> MTDKLIRELLIDVKQKGATRTAKSIENVSDALENAAAASE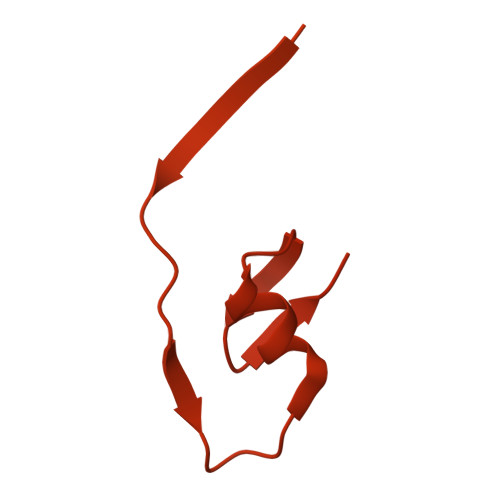LTNEQLGKMPRTLYSIERAADRAAKSLTKMQASRGMAGITKSIDGIGDKLDYLAIQLIEVTDKLEIGFDGVSRSVKAMGNDVAAATEKVQDRLYDTNRALGGTSKGFNDTAGAAGRASRALGNTSGSARGATRDFAAMAKIGGRLPIMYAALASNVFVLQTAFESLKVGDQLNRLEQFGTIVGTMTGTPVQTLALSLQNATNGAISFEEAMRQASSASAYGFDSEQLEQFGLVARRAAAVLGVDMTDALNRVIKGVSKQEIELLDELGVTIRLNDAYENYVKQLNATSTGIKYTVDSLTTYQKQQAYANEVIAESTRRFGYLDDALKATSWEQFAANANSALRSLQQSAATYLNPVMDTLNTFLYQTKSSQMRVSAMARSASAKTTPAENVTALIENAVGAREDLDTYLKESEERVKKAQELKQQLDDLKAKQAATAPIANALTAGGIGGDESNKLVVQLTNELARQNKEIEERTKTEKVLRQAVQDTGEALLRNGKLAEQLGAKMKYADTAVPGDKGVFEVDPNNLKAVSEIQKNFDFLKKSSSDTANNIRMAASSITNAKKASSDLNSVVKAVEDTSKVTGQSADTLVKNLNLGFSSLDQMKAAQKGLSEYVTAMDKSEQNALEVAKRKDEVYNQTKDKAKAEAAAREVLLRQQQEQLTAAKALLAINPNDPEALKQVAKIETEILNTKAQGFENAKKTKDYTDKILGVDREIALLNDRTMTSTQYRLAQLRLELQLEQEKTELYSKQADGQAKVEQSRRAQAQISREIWEAEKQGTASHVSALMDALEVSQTQRNVTGQSQILTERLSILQQQLELSKGNTEEELKYRNEIYKTSAALEQLKKQRESQMQQQVGSSVGATYTPTTGLIGEDKDFADMQNRMASYDQAISKLSELNSEATAVAQSMGNLTNAMIQFSQGSLDTTSMIASGMQTVASMIQYSTSQQVSAIDQAIAAEQKRDGKSEASKAKLKKLEAEKLKIQQDAAKKQIIIQTAVAVMQAATAVPYPFSIPLMVAAGLAGALALAQASSASGMSSIADSGADTTQYLTLGERQKNVDVSMQASSGELSYLRGDKGIGNANSFVPRAEGGMMYPGVSYQMGEHGTEVVTPMVPMKATPNDQLSDGSKTTSGRPIILNISTMDAASFRDFASNNSTAFRDAVELALNENGTTLKSLGNS> GPLGSSFSDFQVLSTLSSTVNSKVYHALRRGEHVAVKEISIDDDAARRRFQREVNIVSTCNHPNIIRIKGVFFDGPFAYILLPYYHRGSLRALLSKQEPMSWVA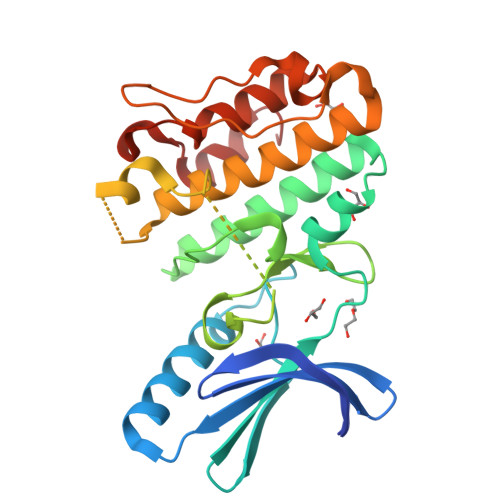VQDMLRQLASGVAYLHEHGIVHGDLKPSNVLIADDGRPVISDFGIAKDHGALGVADMTLTTTVTSTSNGPSSIVGTVQYMAPEQLLCETGSHKTKSTGMSDMWALGFTMLEVALENAFFHDGSLGKPCLPLLLPEQKRIDVPAKAVGGDEKLAEAIASVLVADPGNRATAYDLLAHPYFSS Fungal immunomodulatory proteins (FIPs) are a group of low-molecular-weight (MW) proteins investigated as potential anti-tumor drugs. FIP-nha (from Nectria haematococca) contains two glycosylation sites at positions N5 and N39. In this study, the impact of glycosylation on the bioactivity and biochemical characteristics of FIP-nha (from Nectria haematococca) is described. Taken together, these findings indicate that glycosylation of FIP-nha impacts its thermostability and digestion resistance.

The double-glycosylated wild-type is denominated by WT. However, we only managed to obtain crystals and solved the structures of WT, N39A and N5+39A. Since all structures turned out to be almost identical to each other, we used the structure of the WT as an overall model for the analysis. Specifically, the composition, as analyzed on SDS-PAGE, visualized that the double-glycosylated band of WT represented only 6.7%, while the single glycosylated and un-glycosylated bands accounted for 31.7% and 61.6%, respectively. Unfortunately, none of the structures contained a density indicative of N-glycosylation. The lack of glycosylation in our crystal structures may have been due to the nonuniformity of glycosylated protein or the flexibility of glycan chains. For the simulation, the GlcNAc2Man9 glycan structure was used, as this high mannose-type glycosylation modification is commonly expressed in P. pastoris. Figure 3 shows the obtained crystal structure of WT and its predicted glycosylated form. Based on its crystal structure, N5 is at the start of the N-terminus just in front of the characteristic α-helix and located in the middle of the tetrameric structure. N39 is positioned in the middle of the third β-sheet and located at the four corners of the tetrameric structure. Double glycosylation significantly enhanced the pepsin resistance.

>GPLGSMATTNDSAVLFYIVASQKKLSFDYTPNWGRGSPNSYIDNLTFPRVLTNKPYKYRVVKAGQDLGVRDSYSVQSDGSQKVNFLEYNAGRGIADTQTIQVYVVDPDNGNQYLVAQWKHHHHHH[8x]>MTTSADISLRHVSVLDSTMAYRETGRSDAPVVLFLHGNPTSSYIWRNIIPLVAPVAHCIAPDLIGFGQSGKPDIDYRFFDHVRYLDAFIDKLGIESAYLVAQDWGTALAFHLAARRPDFVRGLAFMEFIRPMPT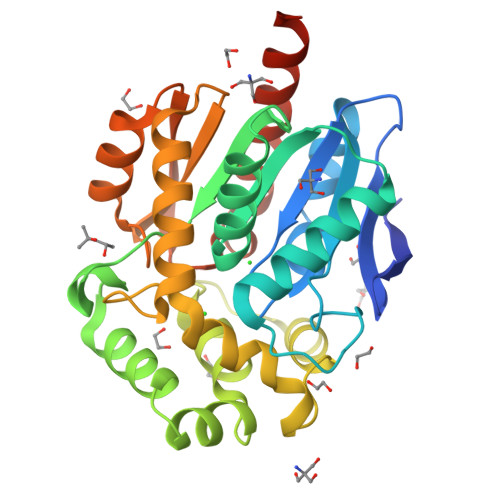WDDFHQTPQAREMFRKFRTPGVGEQMILEDNVFVERVLPGSIVRKLSEEEMAVYRAPFPTPESRRPTLRFPRELPIAGEPADVYSTLESAHAALAASTYPKLLFTGDPGALVSPAFAERFAANLKNCRLIRLGAGLHYLQEDHPEAIGRTVAGWIAEIEAASATAKAHHHHHH[6x]> GGSNPPASPLQDNLVIALHSYEPSHDGDLGFEKGEQLRILEQSGEWWKAQSLTTGQEGFIPFNFVAKANSLEPEPWFFKNLSRKDAERQLLAPGNTHG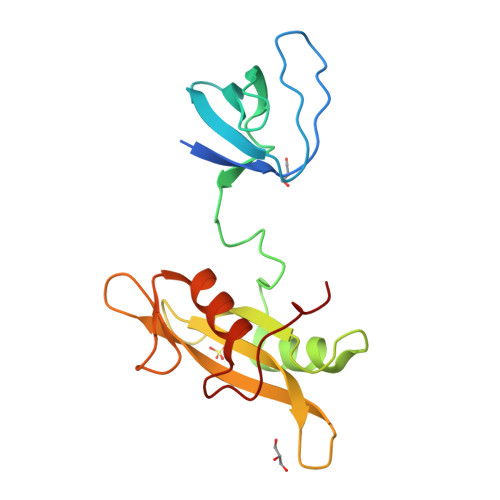SFLIRESESTAGSFSLSVRDFDQNQGEVVKHYKIRNLDNGGFYISPRITFPGLHELVRHYTNASDGLCTRLSRPCQT>[2x]MAPLENNYNESLNKSKDAIDDKTWSKLFPSIVSDPDRSSNFMIRAIYVVFSAVLRQRNILEKEYFSKNYITENLSCMTLSFKNLRAHQIAQLLRAAGDATKDGFLKEISLVVTEHDGDVEAIEVFSMKFIYFENGGVVARLSTDNNDQEDPHFAELAQLRYEGAESVRDQMVTIVR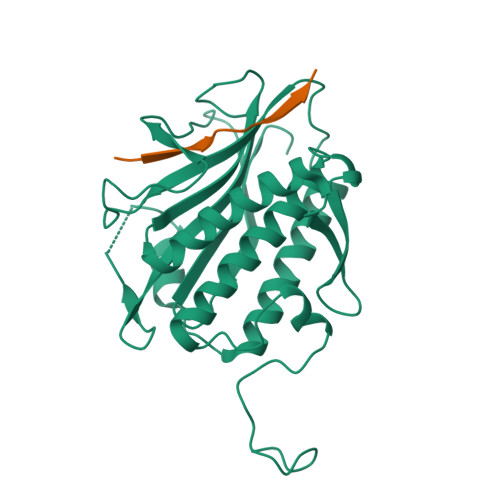SVQFLCTKVLEPLPAEFTANFRLKYTNDAPSNFRIDGFDDSSTFYTLPDGIQSVTIGHLRPGHHAAHMQCWSKSMSD;>[2x]TARYGVSNTSINRKKP> MPGPLGLLCFLALGLLGSAGPSGAAPPLCAAPCSCDGDRRVDCSGKGLTAVPEGLSAFTQALDISMNNITQLPEDAFKNFPFLEELQLAGNDLSFIHPKALSGLKELKVLTLQNNQLKTVPSEAIRGLSALQSLRLDANHITSVPEDSFEGLVQLRHLWLDDNSLTEVPVHPLSNLPTLQALTLALNKISSIPDFAFTNLSSLVVLHLHNNKIRSLSQHCFDGLDNLETLDLNYNNLGEFPQAIKALPSLKELGFHSNSISVIPDGAFDGNPLLRTIHLYDNPLSFVGNSAFHNLSDLHSLVIRGASMVQQFPNLTGTVHLESLTLTGTKISSIPNNLCQEQKMLRTLDLSYNNIRDLPSFNGCHALEEISLQRNQIYQIKEGTFQGLISLRILDLSRNLIHEIHSRAFATLGPITNLDVSFNELTSFPTEGLNGLNQLKLVGNFKLKEALAAKDFVNLRSLSVPYAYQCCAFWGCDSYANLNTEDNSLQDHSVAQEKGTADAANVTSTLENEEHSQIIIHCTPSTGAFKPCEYLLGSWMIRLTVWFIFLVALFFNLLVILTTFASCTSLPSSKLFIGLISVSNLFMGIYTGILTFLDAVSWGRFAEFGIWWETGSGCKVAGFLAVFSSESAIFLLMLATVERSLSAKDIMKNGKSNHLKQFRVAALLAFLGATVAGCFPLFHRGEYSASPLCLPFPTGETPSLGFTVTLVLLNSLAFLLMAVIYTKLYCNLEKEDLSENSQSSMIKHVAWLIFTNCIFFCPVAFFSFAPLITAISISPEIMKSVTLIFFPLPACLNPVLYVFFNPKFKEDWKLLKRRVTKKENLYFQGDYKDDDDKHHHHHHHH

Leucine-rich repeat-containing G protein-coupled receptor 4 (LGR4) plays a critical role in regulating the wingless-related integration site (Wnt) signaling pathway and is essential for organ development and carcinogenesis. LGR4, along with its ligand R-spondin (RSPO), potentiates Wnt/β-catenin signaling by recruiting its signaling suppressor, E3 ligase Zinc and Ring Finger 3 (ZNRF3), and inducing its membrane clearance. Cell surface-expressed LGR4/5, members of the class A G-protein coupled receptors (GPCR) family, have an extracellular domain (ECD) comprising 17 leucine-rich repeats (LRRs), followed by a seven-transmembrane domain (TMD), and an intracellular domain (ICD). ZNRF3/RNF43, LGR4, and RSPO form a ternary complex on the cell surface, which relieves ZNRF3/RNF43-mediated suppression of Wnt/β-catenin signaling and thereby potentiates pathway activation.

We purified lauryl maltose neopentyl glycol/ cholesteryl hemisuccinate (LMNG/CHS) detergent-solubilized human LGR4 (residues 1-822) containing ECD and TMD and determined its structure using cryo-EM to a resolution of 3.5 Å. In the cryo-EM map, the ECD (residues 29-525), TMD (residues 539-822), and connecting segment between the ECD and TMD (residues 526-538) were observed and modeled, except for the extended-loop region at the end of the ECD (residues 476-518). LGR4 ECD adopts a typical horseshoe structure comprising 17 LRRs (residues 58-455) flanked by N-terminal (LRRNT, residues 29-57) and C-terminal (LRRCT, residues 456-525) caps. LGR4 TMD comprises 7-transmembrane (TM) helices typical of GPCRs. LGR4 TMD can be superimposed well on the inactive conformation of the luteinizing hormone-choriogonadotropin receptor (LHCGR/LGR2) with a root-mean-square deviation (RMSD) value of 1.08 Å. Therefore, the GPCR 7-TM structure has an inactive conformation. The ECD was tilted to about 45° relative to the membrane layer, a configuration maintained by interactions at the hinge region between the ECD and TMD, comprising the LRRCT and the following connecting segment. In the upper layer, the LRRCT helix packs complementarily against the extracellular loop (ECL)1 helix from the TMD and the adjacent connecting segment, with the Y468 side chain inserted into a small pocket formed between the ECL1 helix and the connecting segment. In the lower layer, the connecting segment formed a three-successive-turn structure that interacted extensively with the presumed ligand-binding pocket on the extracellular side of the TMD. In the inactive conformation of LGR4, F529, F696, and M782 blocked the entrance to the pocket; however, the structural transition from the inactive to the active state may allow the pocket to widen, as observed in LGR2, enabling it to accommodate such ligands.> MVDAVVTVFLEKTLNILEEKGRTVSDYRKQLEDLQSELKYMQSFLKDAERQKRTNETLRTLVADLRELVYEAEDILVDCQLADGDDGNEQRSSNAWLSRLHPARVPLQYKKSKRLQEINERITKIKSQVEPYFEFITPSNVGRDNGTDRWSSPVYDHTQVVGLEGDKRKIKEWLFRSNDSQLLIMAFVGMGGLGKTTIAQEVFNDKEIEHRFERRIWVSVSQTFTEEQIMRSILRNLGDASVGDDIGTLLRKIQQYLLGKRYLIVMDDVWDKNLSWWDKIYQGLPRGQGGSVIVTTRSESVAKRVQARDDKTHRPELLSPDNSWLLFCNVAFAANDGTCERPELEDVGKEIVTKCKGLPLTIKAVGGLLLCKDHVYHEWRRIAEHFQDELRGNTSETDNVMSSLQLSYDELPSHLKSCILTLSLYPEDCVIPKQQLVHGWIGEGFVMWRNGRSATESGEDCFSGLTNRCLIEVVDKTYSGTIITCKIHDMVRDLVIDIAKKDSFSNPEGLNCRHLGISGNFDEKQIKVNHKLRGVVSTTKTGEVNKLNSDLAKKFTDCKYLRVLDISKSIFDAPLSEILDEIA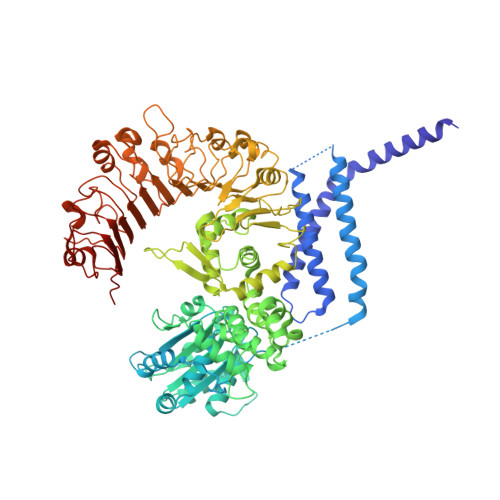SLQHLACLSLSNTHPLIQFPRSMEDLHNLQILDASYCQNLKQLQPCIVLFKKLLVLDMTNCGSLECFPKGIGSLVKLEVLLGFKPARSNNGCKLSEVKNLTNLRKLGLSLTRGDQIEEEELDSLINLSKLMSISINCYDSYGDDLITKIDALTPPHQLHELSLQFYPGKSSPSWLSPHKLPMLRYMSICSGNLVKMQEPFWGNENTHWRIEGLMLSSLSDLDMDWEVLQQSMPYLRTVTANWCPELESFAIEDVGFRGGVWMKTPLHRT>MDSGDGQDLRAFVHDSPEETETTQRLTKLLTNSPIPTEELVNNLPLFLRRHQMTDLLSMDALYRQVLDVPGVIMEFGVRFGRHLGTFAALRGVYEPYNPLRRIVGFDTFTGFPDVNDVDRVGPTAYQGRFAVPGGYPAYLKEVLDAHEC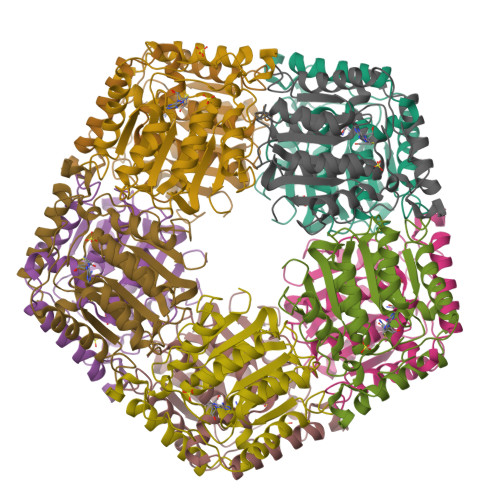SDFFGHVTQRSVLVEGDVRETVPRYLAENPQTVIALAYFDLDLYEPTKAVLEAIRPYLTKGSIVAFDELDNPKWPGENIAMRKVLGLDHAPLRLLPGRPAPAYLRWGD[20x]>[7x]MSVPTVLQKILARKAEEVAERRARVNLAEVERLARSADAPRGFANALLERAKRKEPAVIAEIKKASPSKGVLREH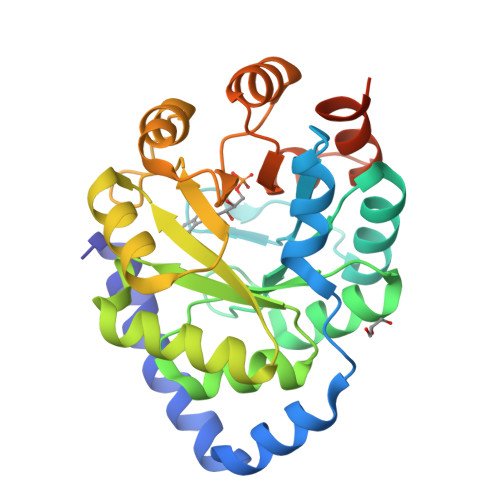FVPAEIARSYEAGGAACLSVLTDVDFFQGADAYLKEARAACALPVIRKDFMIDPYQIVEARAIGADCILLIVSALDDVLMAELAATAKSVGLDVLVEVHDGTELERALKTLDTPLVGINNRNLHTFEVSLETTLDLLPEIPRDRLVVTESGILNRADVELMEVSEVYAFLVGEAFMRADDPGLELKRLFFQERGAVVLGADPDTSGHHHHHH;> XXXXXXXXXXXXXXVNLAEVERLARSADAPRGFANALLERAKRKEPAVIAEIKKASPSKGVLREHFVPAEIARSYEAGGAACLSVLTDVDFFQGADAYLKEARAACALPVIRKDFMIDPYQIVEARAIGADCILLIVSALDDVLMAELAATAKSVGLDVLVEVHDGTELERALKTLDTPLVGINNRNLHTFEVSLETTLDLLPEIPRDRLVVTESGILNRADVELMEVSEVYAFLVGEAFMRADDPGLELKRLFFQERGAVVLGADPDTSGHHHHHH> GAMGSRQWALEDFEIGRPLGKGKF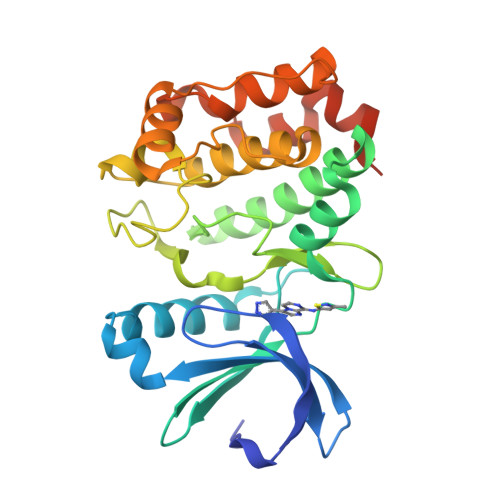GNVYLAREKQSKFILALKVLFKAQLEKAGVEHQLRREVEIQSHLRHPNILRLYGYFHDATRVYLILEYAPLGTVYRELQKLSKFDEQRTATYITELANALSYCHSKRVIHRDIKPENLLLGSAGELKIADFGWSVHAPSSRRAALCGTLDYLPPEMIEGRMHDEKVDLWSLGVLCYEFLVGKPPFEANTYQETYKRISRVEFTFPDFVTEGARDLISRLLKHNPSQRPMLREVLEHPWITANSSKPSNCQNKESASKQS>[2x]GSHMGEIRPTIGQQMETGDQRFGDLVFRQLAPNVWQHTSYLDMPGFGAVASNGLIVRDGGRVLVVDTAWTD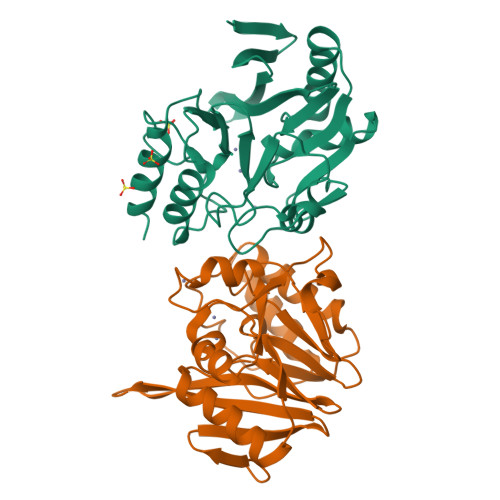DQTAQILNWIKQEINLPVALAVVTHAHQDKMGGMDALHAAGIATYANALSNQLAPQEGMVAAQHSLTFAANGWVEPATAPNFGPLKVFYPGPGHTSDNITVGIDGTDIAFGGCLIKDSKAKSLGNLGDADTEHYAASARAFGAAFPKASMIVMSHSAPDSRAAITHTARMADKLR> MNLPTAQEVQGLMARYIELVDVGDIEAIVQMYADDATVEDPFG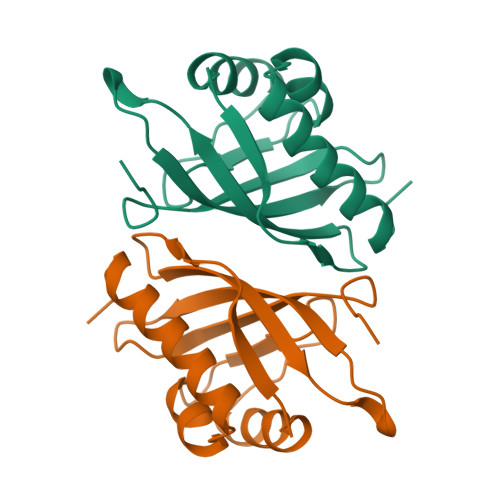QPPIHGREQIAAFYRQGLGGGKVRACLTGPVAASHNGCGAMPFRVEMVWNGQPCALDVIDVMRFDEHGRIQTMQAYWSEVNLSVREPQ>[2x]MSGRVGDLSPRQKEALAKFRENVQDVLPALPNPDDYFLLRWLRARSFDLQKSEAMLRKHVEFRKQKDIDNIISWQPPEVIQQYLSGGMCGYDLDGCPVWYDIIGPLDAKGLLFSASKQDLLRTKMRECELLLQECAHQTTKLGRKVETITIIYDCEGLGLKHLWKPAVEAYGEFLCMFEENYPETLKRLFVVKAPKLFPVAYNLIKPFLSEDTRKKIMVLGANWKEVLLKHISPDQVPVEYGGTMTDPDGNPKCKSKINYGGDIPRKYYVRDQVKQQYEHSVQISRGSSHQVEYEILFPGCVLRWQFMSDGADVGFGIFLKTKMGERQRAGEMTEVLPNQRYNSHLVPEDGTLTCSDPGIYVLRFDNTYSFIHAKKVNFTVEVLLPDKASEEKMKQLGA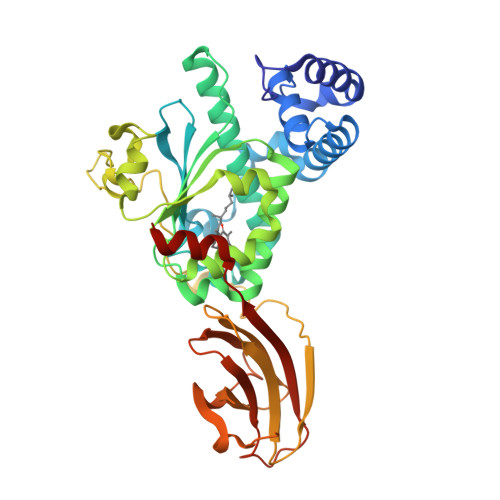GTPK;> MSGRVGDLSPRQKEALAKFRENVQDVLPALPNPDDYFLLRWLRARSFDLQKSEAMLRKHVEFRKQKDIDNIISWQPPEVIQQYLSGGMCGYDLDGCPVWYDIIGPLDAKGLLFSASKQDLLRTKMRECELLLQECAHQTTKLGRKVETITIIYDCEGLGLKHLWKPAVEAYGEFLCMFEENYPETLKRLFVVKAPKLFPVAYNLIKPFLSEDTRKKIMVLGANWKEVLLKHISPDQVPVEYGGTMTDPDGNPKCKSKINYGGDIPRKYYVRDQVKQQYEHSVQISRGSSHQVEYEILFPGCVLRWQFMSDGADVGFGIFLKKKMGERQRAGEMTEVLPNQRYNSHLVPEDGTLTCSDPGIYVLRFDNTYSFIHAKKVNFTVEVLLPDKASEEKMKQLGAGTPK>[2x]MT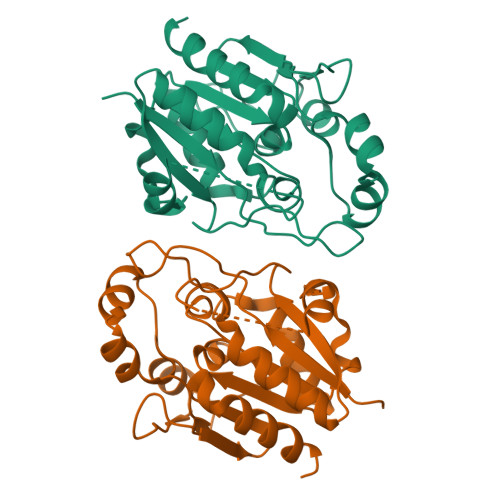PKRALISLTSYHGPFYKDGAKTGVFVVEILRSFDTFEKHGFEVDFVSETGGFGWDEHYLPKSFIGGEDKMNFETKNSAFNKALARIKTANEVNASDYKVFFASAGHGALFDYPKAKNLQDIASKIYANGGVIAAICHGPLLFDGLIDIKTTRPLIEGKAITGFPLEGEIALGVDDILRSRKLTTVERVANKNGAKYLAPIHPWDDYSITDGKLVTGVNANSSYSTTIRAINALYSVEHHHHH>SGGGDGSTYSAEIRRTTMGVPHIKAGNWGSAGYGFGYVQAQDNLCTMADSFLTYRGERSRHLGGSAQLVYNSTLGRPRNIDSDFFHRHVISDEAVDRTMAAQPAKLLQMVEGFAAGYNRYVREAKAGGSAHAACRSEAWVQPITARDVWR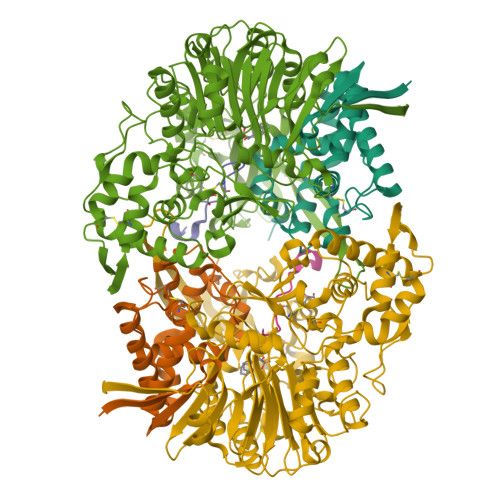RIYAANLAGGYSNFAEAIANAQPPQAKA[4x];>GAQEPAAFEPGRTRAPSLQVGGELGVG[4x];>[4x]SNMYGFGTAATGEGSGVLFGNPHWYWKGPDRFYQAQLTIDGEANVSGVSFLGLPVIQIGFNDSVAWSHTVSTARRFGFFQLSLVQGEPTSYLRDGVPVKMKPATITVPSRNADGSVSDVTRTLYHSEFGPLVNLAGLNPALAWSQGTAFAIRDINGENFRTLRTWMRWNQAKSLDEFIAIQKEEASIPWVNTVAVGRGSAKAWYADIGAVPNVSPAQTAACTTPFGMAVGQALPNVPFFDGSRSECDWLTDADSVQKGAVGVSRMPSLQRDDYVGNMNDSYWLANVHAPLTGYPAIFGPAGTSAQTLRTRMGHTMALERLAGTDGYAGNKATSAVVREMVLGSRVFSAERFKDEVLDLICTPAQWTVNGAAVDAAQACAVLAAWDNRGRKDSRGSHLWDEFWSRVPTASLFTVPFSAADPLNTPRGINAAAADALRQAMATAIARVGQSGYALDAPRGEVLYATRGGTRLPLYGGCGAMGYFTITCSENDITQGGYSMDGQPNASNSYMQVVSFPASGVQAHTFLTFSLSDDPASPHHGDYTKAYSAGQWLRVPFTEAEITGNADYRTATVKELEHHHHHH>GPRQWALEDFEIGRPLGKGKFGNVYLAREKQSKFILALKVLFKAQLEKAGVEHQLRREVEIQSHLRHPNILRLYGYFHDATRVYLILEYAPLGTVYRELQKLSKFDEQRTATYIT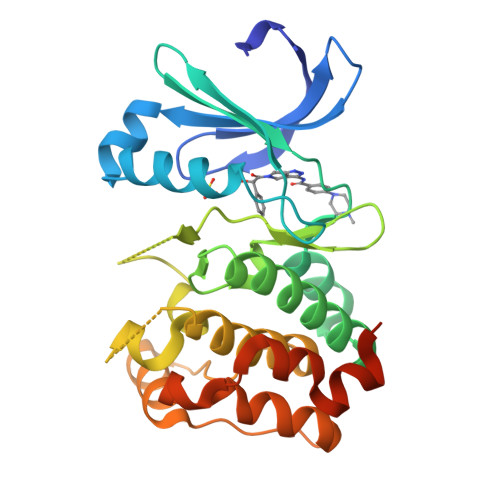ELANALSYCHSKRVIHRDIKPENLLLGSAGELKIADFGWSVHAPSSRRTTLCGTLDYLPPEMIEGRMHDEKVDLWSLGVLCYEFLVGKPPFEANTYQETYKRISRVEFTFPDFVTEGARDLISRLLKHNPSQRPMLREVLEHPWITANSSKPSNCQNKESASKQS[2x]> QNSETGALKTFITQQGIKSQHQTKEEQSQITSQVTGQIGWRREGIKYRRNELFLDVLESVNLLMSPQGQVLSAHVSGRVVMKSYLSGMPECKFGMNDKIVIEKQGKGTADETSKSGKQSIAIDDCTFHQCVRLSKFDSERSISFIPPDGEFELMRYRTTKDIILPFRVI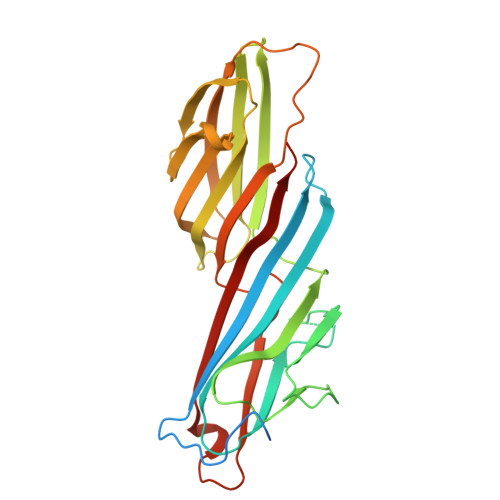PLVREVGRTKLEVKVVIKSNFKPSLLAQKIEVRIPTPLNTSGVQVICMKGKAKYKASENAIVWKIKRMAGMKESQISAEIELLPTNDKKKWARPPISMNFEVPFAPSGLKVRYLKVFEPKLNYSDHDVIKWVRYIGRSGIYETRC> HMRDEILDPSNLVKNREILY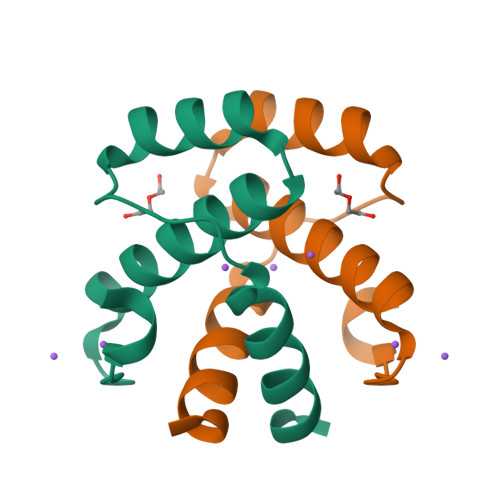RLMISQLMYDGLEKFAMELSMLVKADQCAPSERLLHVMIAGMQTLS>MGNLYSSLPLTKREEVEKLLN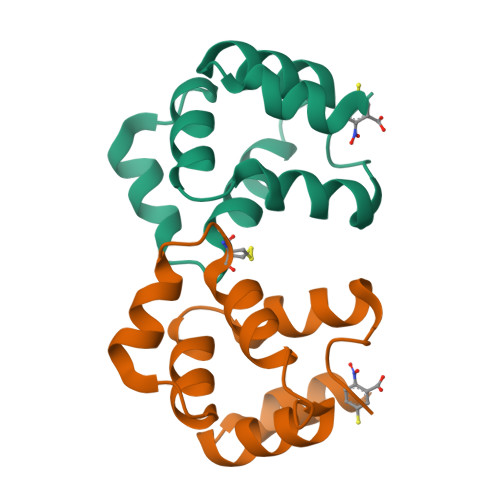GDTWRHLAGELGYQPEHIDSFTHEACPVRALLASWGAQDSATLDALLAALRRIQRADIVESLCSELEHHHHHH[2x]>ASHHLRMHFKTLPAGESLGSLGLWVWGDVDQPSKDWPNGAITMTKAKKDDYGYYLDVPLAAKHRQQVSY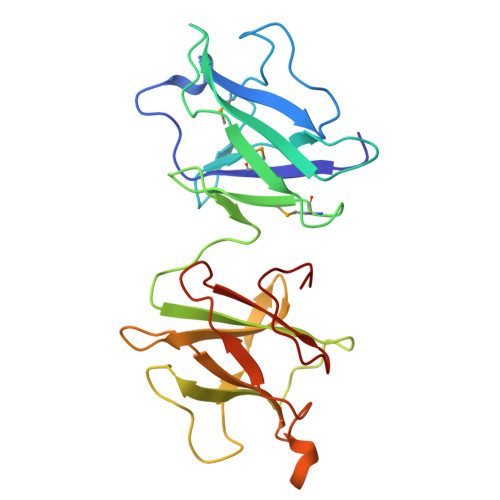LINNKAGENLSKDQHISLLTPKMNEVWIDENYHAHAYRPLKEGYLRINYHNQSGHYDNLAVWTFKDVKTPTTDWPNGLDLSHKGHYGAYVDVPLKEGANEIGFLILDKSKTGDAIKVQPKDYLFKELDNHTQVFVKDTDPKVYNNPYYID[2x]>MGSSHHHHHHQQKLTSPDNNLVMTFQVDSKGAPTYELTYKNKVVIKPSTLGLELKKEDNTRTDFDWVDRRDLTKLDSKTNLYDGFEVKDTQTATFDETWQPVWGEEKEIRNHYNELAVTLYQPMNDRSIVIRFRLFNDGLGFRYEFPQQKSLNYFVIKEEHSQFGMNGDHIAFWIPGDYDTQEYDYTISRLSEIRGLMKEAITPNSSQTPFSQTGVQTALMMKTDDGLYINLHEAALVDYSCMHLNLDDKNMVFESWLTPDAKGDKGYMQTPCNTPWRTIIVSDDARNILASRITLNLNEPCKIADAASWVKPVKYIGVWWDMITGKGSWAYTDELTSVKLGETDYSKTKPNGKHSANTANVKRYIDFAAAHGFDAVLVEGWNEGWEDWFGNSKDYVFDFVTPYPDFDVKEIHRYAARKGIKMMMHHETSASVRNYERHMDKAYQFMADNGYNSVKSGYVGNIIPRGEHHYGQWMNNHYLYAVKKAADYKIMVNAHEATRPTGICRTYPNLIGNESARGTEYESFGGNKVYHTTILPFTRLVGGPMDYTPGIFETHCNKMNPANNSQVRSTIARQLALYVTMYSPLQMAADIPENYERFMDAFQFIKDVALDWDETNYLEAEPGEYITIARKAKDTDDWYVGCTAGENGHTSKLVFDFLTPGKQYIATVYADAKDADWKENPQAYTIKKGILTNKSKLNLHAANGGGYAISIKEVKDKSEAKGLKRL[2x]

Here we describe the three-dimensional structure and mechanistic characterization of the enzyme encoded by susB, a GH97 α-glucosidase from B. thetaiotaomicron (BtGH97a). BtGH97a was shown to hydrolyze a range of substrate sizes from maltose to maltoheptaose, and both α-1,4 and α-1,6 linkages. The tertiary structure of BtGH97a reveals three domains; an N-terminal β-super-sandwich domain (residues 1–317), followed by a canonical (β/α)8 barrel (residues 318–636) and a C-terminal β sheet domain (residues 637–738). The three-dimensional structure and kinetic analyses of BtGH97a reveal an unusual calcium ion-dependent catalytic center in which a glutamate residue is poised to activate the nucleophilic water molecule with both general acid and calcium ion assistance to leaving group departure.

The inhibition of BtGH97a using classical α-glycosidase inhibitors yielded Ki values of 59 μM for deoxynojirimycin 1, 59 μM for castanospermine 2, and 108 nM for acarbose 3. The structures of BtGH97a in complex with 1 and 2 were determined at 1.7 and 2.0 Å resolution, respectively. Clear 2Fobs − Fcalc electron density in the active site (of both molecules of the asymmetric unit) allowed facile building of the complexes. Both 1 and 2 are found in a slightly flattened (toward 4E) 4C1 chair conformation. Each of the inhibitors and the surrounding active-site residues superpose perfectly, so only the interactions for BtGH97a in complex with 1 are described. Hydrogen bonds are formed between the hydroxyl group at C6 and Glu439, between the hydroxyl at C4 and Glu391 and Trp331, and between the hydroxyl at C3 and Lys467. The hydroxyl group at the C2 position interacts with the calcium ion and with His507. The ring nitrogen atom of 1 interacts with a water molecule, which is also within hydrogen bonding distance of Glu439 and Glu508, and hence may mimic the catalytic water molecule in an inverting mechanism (described below in light of 1H NMR experiments). The calcium ion assumes an octahedral coordination, with six ligands, as was observed in the native structure. It coordinates the same four glutamate residues (Glu194, Glu508, Glu526, and Glu532), but instead of interacting with an ethylene glycol molecule, it now coordinates the hydroxyl group at C2 of 1 and a water molecule (all at a distance of between 2.3 and 2.5 Å).>GSHSEADNYARELKREQEEIIRVPDTEAAEVAEILARYGIEPHEYGPVVNALRKKPQAWLDFMMKFELGLEKPDPKRAL[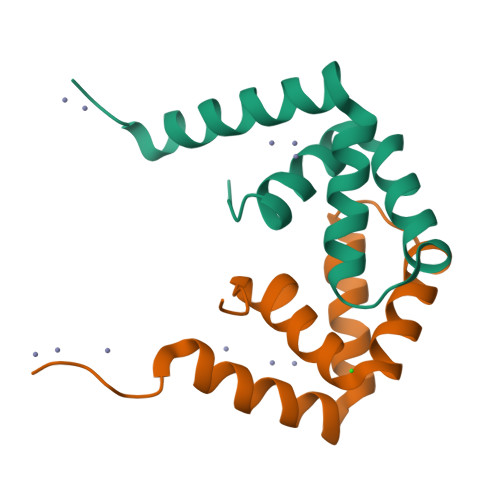8x]>[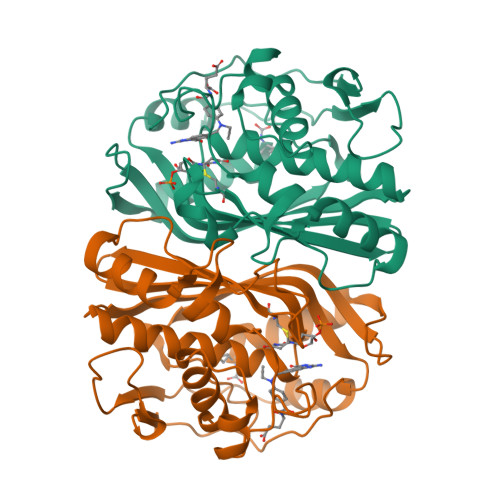6x]MKQYLELMQKVLDEGTQKNDRTGTGTLSIFGHQMRFNLQDGFPLVTTKRCHLRSIIHELLWFLQGDTNIAYLHENNVTIGDEWADENGDLGPVYGKQWRAWPTPDGRHIDQITTVLNQLKNDPDSRRIIVSAWNVGELDKMALAPCHAFFQFYVADGKLSCQLYQRSCDVFLGLPFNIASYALLVHMMAQQCDLEVGDFVWTGGDTHLYSNHMDQTHLQLSREPRPLPKLIIKRKPESIFDYRFEDFEIEGYDPHPGIKAPVAI2,2'-[(2-{[2-({[(2S,3S,4R,5R)-5-(2,4-dioxo-3,4-dihydropyrimidin-1(2H)-yl)-3,4-dihydroxytetrahydrofuran-2-yl]carbonyl}amino)ethyl]amino}-2-oxoethyl)imino]diacetic acid (non-preferred name) | C17 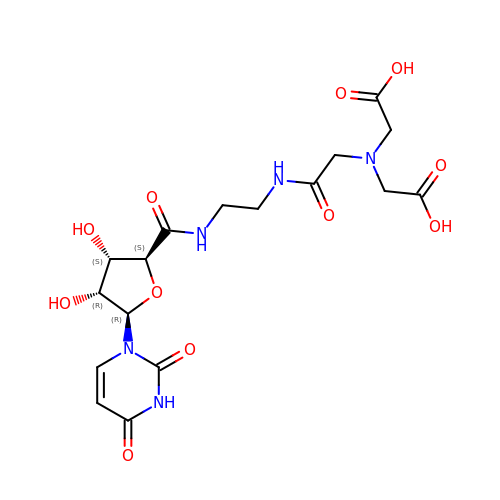H23 N5 O11 | YIXIGZCQDCRABL-KNCOVGOOSA-N2-(3-hydroxyphenyl)-N-(pyridin-2-yl)acetamide | C13 H12 N2 O2 | 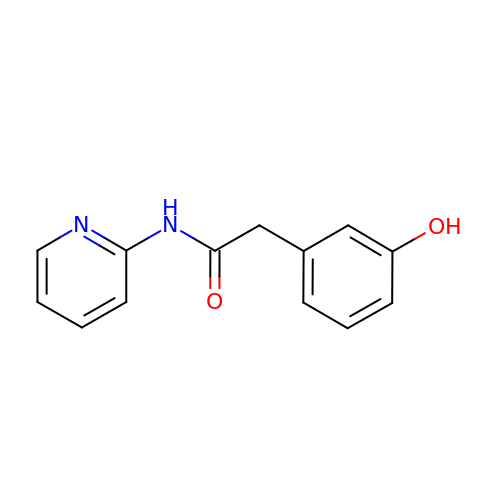XKXNXBRQAPWSNN-UHFFFAOYSA-N> MDAVIKVIGVGGGGGNAVEHMVRERIEGVEFFAVNTDAQALRKTAVGQTIQIGSGITKGLGAGANPEVGRNAADEDRDALRAALEGADMVFIAAGMGGGTGTGAAPVVAEVAKDLGILTVAVVTKPFNFEGKKRMAFAEQGITELSKHVDSLITIPNDKLLKVLGRGISELDAFGAANDVLKGAVQGIAELITRPGLMNVDFADVRTVMSEMGYAMMGSGVASGEDRAEEAAEMAISSPLLEDIDLSGARGVLVNITAGFDLRLDEFETVGNTIRAFASDNATVVIGTSLDPDMNDELRVTVVATGIG

FtsZ, a bacterial homolog of tubulin, assembles onto a ring-like scaffold called the Z-ring, which serves as the foundation for cell division by the divisome. The N-terminal subdomain contains the binding site for GTP, and the C-terminal subdomain has, by analogy with tubulin protofilaments, key catalytic residues that contact the GTP in the subunit below to initiate GTP hydrolysis. Strikingly, although E. coli has provided the most detailed understanding of the machinery and mechanism of bacterial cell division, the structure of the E. coli FtsZ (EcFtsZ) protein has remained elusive. Here, we report the 1.35 and 1.40 Å resolution structures of E. coli FtsZ(L178E) bound to GDP and GTP, respectively.

Du and coworkers focused on one mutant, L178E, which they confirmed to be assembly-incompetent in the presence of GTP. They also found that EcFtsZ(L178E) lost its tendency to aggregate when bound to GDP, as determined by size-exclusion chromatography. The EcFtsZ(L178E) protein, which previous studies had indicated to be a monomer in the presence of GDP or GTP, produced well diffracting crystals in the presence of GDP and, when optimized, permitted us to collect data to 1.35 Å resolution. One clear solution was obtained, consistent with the presence of one EcFtsZ(L178E) molecule in the crystallographic asymmetric unit. In spite of evidence that the L178E mutation in EcFtsZ inhibits assembly, the crystals showed that EcFtsZ(L178E) assembled into straight protofilaments, as noted in the previous study of Du et al.. However, comparison of the EcFtsZ(L178E) filament with the SaFtsZ filament reveals that the EcFtsZ filament is much looser (see below for the buried surface areas). While the residues in the EcFtsZ(L178E) loops from residues 63 to 70 and 168 to 178 make somewhat similar interactions with neighboring subunits to those observed in the SaFtsZ filament, they are more surface-exposed in the EcFtsZ(L178E) crystal filament and their relatively high B factors (the average B factors for residues 63–70 and residues 168–178 are 56.9 and 45.5 Å2, respectively, compared with the overall average protein B factor of 23.9 Å2) indicate they are somewhat flexible. Presumably, as the residue corresponding to Leu178 in SaFtsZ is wedged into a hydrophobic pocket of an adjacent subunit in the SaFtsZ filament, the similar burial of the Glu178 side chain into the hydrophobic pocket in the EcFtsZ(L178E) filament is predicted to be unfavorable. As a result, the EcFtsZ(L178E) protofilaments have a more open subunit interface. Our analyses show that the EcFtsZ(L178E) structure adopts the R state and as such has a closed cleft between its N-terminal and C-terminal subdomains.>[8x]MRKIVVAAIAVSLTTVSITASASADPSKDSKAQVSAAEAGITGTWYNQLGSTFIVTAGADGA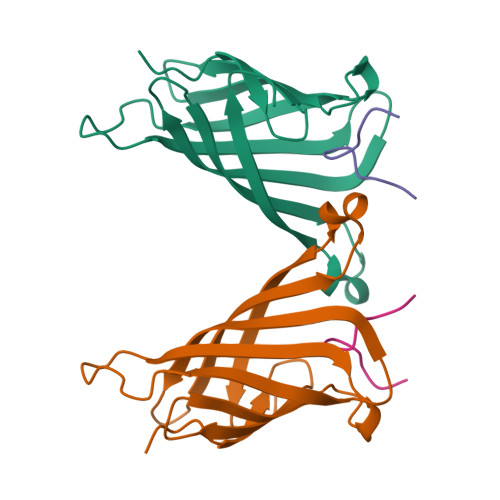LTGTYESAVGNAESRYVLTGRYDSAPATDGSGTALGWTVAWKNNYRNAHSATTWSGQYVGGAEARINTQWLLTSGTTEANAWKSTLVGHDTFTKVKPSAASIDAAKKAGVNNGNPLDAVQQ;>[8x]EWVHPQFEQKAK> MHHHHHHHHHHHHLPPITPQELESMSPQEQRAALGDRLFLKVYEIAPELAPKITGMFLEMKPKEAYELL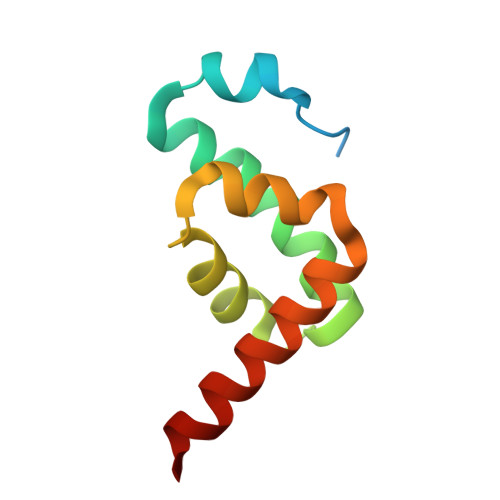NDQKRLEERVTEALCVLKAHQTA> LTSLPNRAFFEGRLSRALRDANEHREQLAVLFIDSDRFKEINDRLGHAAGDTVLVNIAMRIRGQLRESDLVARLGGDEFAVLLAPLASGADALRIADNIIASMQAPIRLSDGSTVSTSLTIGIALYPEHADTPAALLHDADMAMYIAKRQARGSRRLAELN

YfiN, also called TpbB, is a multi-domain membrane enzyme connecting periplasmic stimuli to cytosolic c-di-GMP production by an allosteric inside-out signaling mechanism that, due to the lack of structural data, is still largely hypothetical. YfiN is an inner membrane protein composed of three domains: a periplasmic PAS domain, two transmembrane helices and a cytosolic portion of the protein, which includes an HAMP domain and a cyclase domain (named GGDEF from the conserved residues in the active site). Formation of SCVs depends on enhanced c-di-GMP output by YfiN, which elevates transcription of the pel operon. The negative regulator YfiR is a dimeric periplasmic protein which controls the activity of YfiN by binding to the PAS domain of the DGC.

In order to gain structural insights on the allosteric regulation of YfiN, we expressed the cytosolic portion of the protein, including the HAMP and the GGDEF cyclase domain (YfiNHAMP-GGDEF; residues 183-435). The solved structure confirmed that YfiNHAMP-GGDEF had actually undergone proteolysis and that only the GGDEF domain had crystallized (YfiNGGDEF). The crystal structure of the catalytic domain of YfiN is composed by a five-stranded β-sheet core (β2-3-1-6-7) flanked by five α-helices (αA to F). YfiNGGDEF also displays an additional peripheral β-hairpin (β4-5), which is present in all the homologues structures (PleD from Caulobacter crescentus; WspR from P. aeruginosa; XCC4471 from Xanthomonas campestris and A1U3W3 from Marinobacter aquaeolei) with the exception of WspR that displays a long loop in a very different conformation. However, the cyclase domain of YfiN significantly differs from the other homologues at the level of the allosteric inhibitory site (I-site). The GGDEF domain of YfiN displays a conserved RxxD motif in the Ip , while the Is appears degenerated. In particular, the second arginine necessary to form an inactive GGDEF/GGDEF dimer, is substituted with Asp-273. Finally, the α-helix harboring the Is (α-A) is shifted with respect to the corresponding helix of PleD, WspR and A1U3W3, which all display product feedback inhibition. The shift is due to the hindrance of Tyr-379 side chain.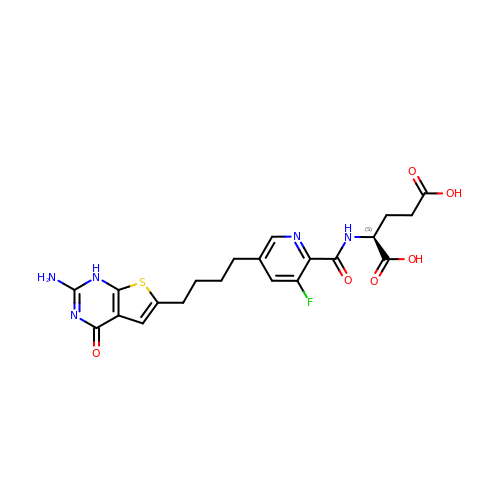N-{5-[4-(2-amino-4-oxo-1,4-dihydrothieno[2,3-d]pyrimidin-6-yl)butyl]-3-fluoropyridine-2-carbonyl}-L-glutamic acid | C21 H22 F N5 O6 S | USGRXMVHCFOWQP-AWEZNQCLSA-N> MTDNHIDVLINGCGIGGAMLAYLLGRQGHRVVVVEQARREYARNRADLLKPAGIRVVEAAGLLAEVTRRGGRVRHELEVYHDGELLRYFNYSSVDARGYFILMPGESLRRLVLEKIDGEATVEMLFETRIEAVQRDERHAIDQVRLNDGRVLRPRVVVGADGIASYVRRRLLDIDVERRPYPSPMLVGTFALAPCVAERNRLYVDSQGGLAYFYPIGFDRARLVVSFPREEARELMADTRGESLRRRLQRFVGDESAEAIAAVTGTSRFKGIPIGYLNLDRYWADNVAMLGDAIHNVHPITGQGMNLAIEDASALADALDLALRDACALEDALA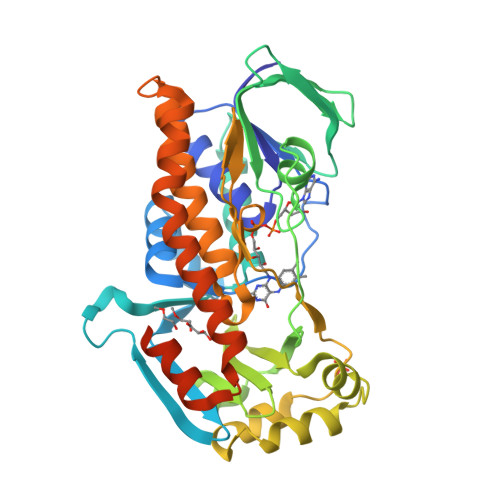GYQAERFPVNQAIVSYGHALATSLEDRQRFAGVFDTALQGSSRTPEALGGERSYQPVRSPAPLG> KIQVKCSAPNSVTITNASGGLYLVEYPEGYVAYSKATEVTGKLVHANFGTKKDFEDL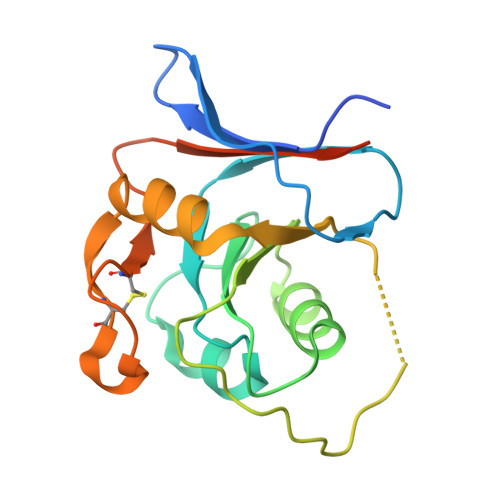DYAVNGSIVIVRAGKITIAEKVANAQSFNAIGVLIYKDRTKYPISRADEPLQGHSGLPSIPVQTISREAAEKLFQNMERDCPRSWNTDSSCKLELLQNRNVKLTVNNCLKEGTSGHHHHHH> MYRSTKGASKARRDQINAEIRNLKELLPLAEADKVRLSYLHIMSLACIYTRKGVFFAGGTPLAGPTGLLSAQELEDIVAALPGFLLVFTAEGKLLYLSESVSEHLGHSMVDLVAQGDSIYDIIDPADHLTVRQQLTMPSALDADRLFRCR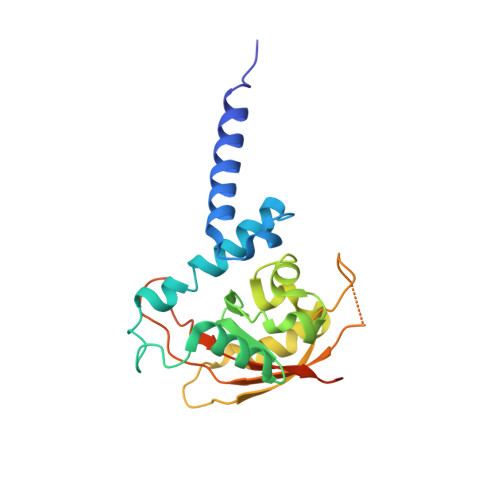FNTSKSLRRQSSGNKLVLIRGRFHAHPPGAYWAGNPVFTAFCAPLEPRPRPGPGPHHHHHH> MIGVNRMTEASTYIGTVQDVNGANIRVVLDINTISSLKFVDGQGYRIGQIGSFVRIPIGYINLFGIVSQVGAGAVPDKLLEVEPYGHRWISVQLVGEEGIKKEFERGVSQYPTIGDKVHIVTEPDLKKIYGTQNKKYISLGNIASVDSIPALVNIDTLVTRHSAVLGSTGSGKSTTVTSILQRISDMSQFPSARIIVFDIHGEYAAAFKGKAKVYKVTPSNNELKLSIPYWALTCDEFLSVAFGGLEGSGRNALIDKIYELKLQTLKRQEYEGINEDSLTVDTPIP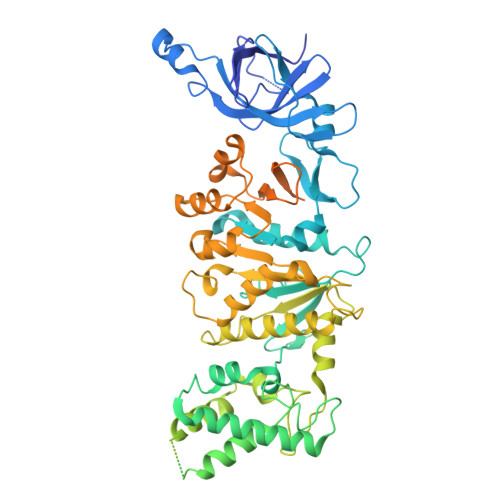FSIHKLWFDLYRAEISTHYVQGSHSEENEALLLGEDGNPVQKGDSLKVVPPIYMPHTQAQGATKIYLSNRGKNIRKPLEGLASLLKDPRYEFLFNADDWSVNLDGKTNKDLDALLETWVGSEESISIFDLSGMPSSILDTLIGILIRILYDSLFWSRNQPEGGRERPLLVVLEEAHTYLGKDSRGIAIDGVRKIVKEGRKYGIGMMLVSQRPSEIDSTILSQCGTLFALRMNNSSDRNHVLGAVSDSFEGLMGMLPTLRTGEAIIIGESVRLPMRTIISPPPFGRRPDSLDPDVTAKWSNNRVQGDYKEVLTLWRQKKVRSQRIVENIKRLPVVNEGEMTDMVREMVTSSNILSIGYEADSMTLEIEFNHGLVYQYYDVPETLHTELLAAESHGKFFNSQIKNNYRFSRI> AGKNVNVEFRKGHSSAQYSGEIKGYDYDTYTFYAKKGQKVHVSISNEGADTYM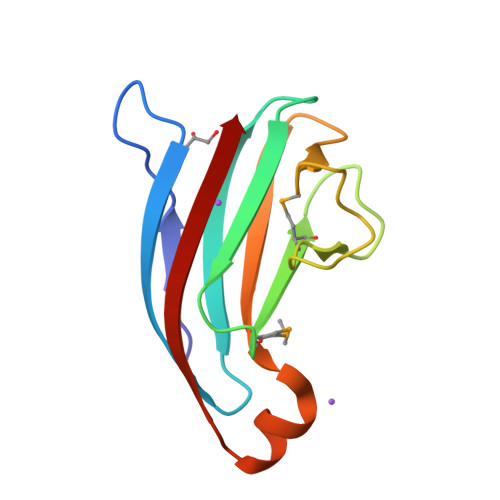FGPGIDDSVDLSRYSPELDSHGQYSLPASGKYELRVMQTRNDARKNKTKKYNVDIQIK>MMKPEDVIKEQCARAKVVAELWHGFTGGAPKAALENLVVEFNKAQQGRCVRPVPQGGFRDLSTKIKAAFAAGKVPTMAQAFENNIALYLEAKALLPIESLGVKLQGVNLTFLNAVRFGGVVYGVPFNKSIQVLYYNKDLLKKHGVPVPATLEEFVAAAKKLSRAEGGPVYWFQPDASTFAYFFFNLGGSYLKDGKLVLNSKEAVEALTLLQNGVKEGWAKPITSGYINQNLGSGPYAFSVDTSAGYTYYLRAAKFDLGVATLPGRTKGQPGYGLVQGTNLVVFRQASKEEQAVAKDFLE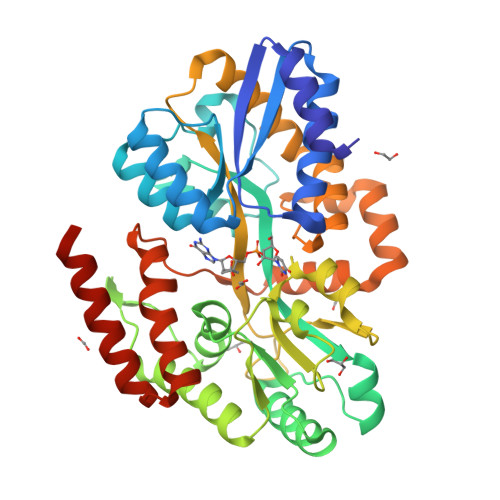FVLSPRAQAVFATATGYVPVTEGALKDPVYQAYAAENPDYATIVRQSRYAKFEPALAEWEQIRFDILGQAIKEAILNKADPKAALDRAQKLAEDLLSSRTRHHHHHH[2x]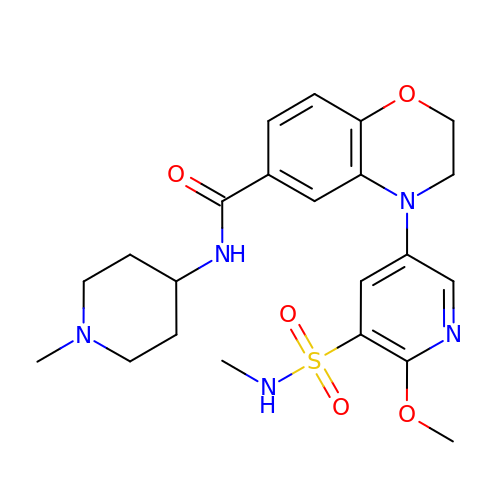4-[6-methoxy-5-(methylsulfamoyl)pyridin-3-yl]-~{N}-(1-methylpiperidin-4-yl)-2,3-dihydro-1,4-benzoxazine-6-carboxamide | C22 H29 N5 O5 S | NNWATAZUOWDGHZ-UHFFFAOYSA-N> GACCAAUCUGCCCUCAGAGCUCGAGAACAUCUUCGGAUGCAGAGGAGGCAGGCUUCGGUGGCGCGAU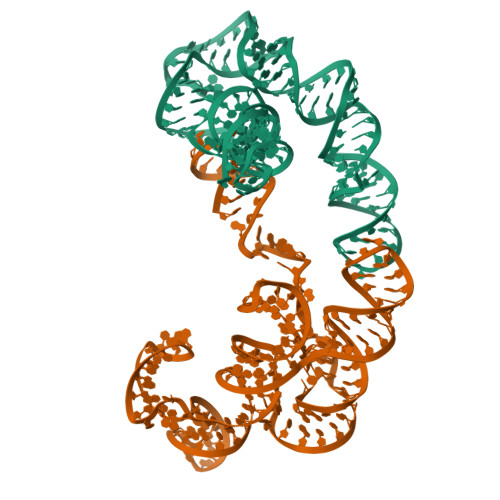AGCGCCAACGUCCUCAACCUCCAAUGCAUCCCACCACAUGAUGAUGCCUGAAGAGCCUUGGUUUUUUG;> GGAUCUUCUCGAUCUAACAAAAAAGACAAAUCUGCCACAAAGCUUGAGAGCAUCUUCGGAUGCAGAGGCGGCAGCCUUCGGUGGCGCGAUAGCGCCAACGUUCUCAACUAUGACACGCAAAACGCGUGCUCCGUUGAAUGGAGUUUAUCAUG> EDKIMSYNAFFWMWVHDMLIDSIKWRDEHGRCINKDKGKTCIKGCNKKCISFQKWVEQKKTEWGKI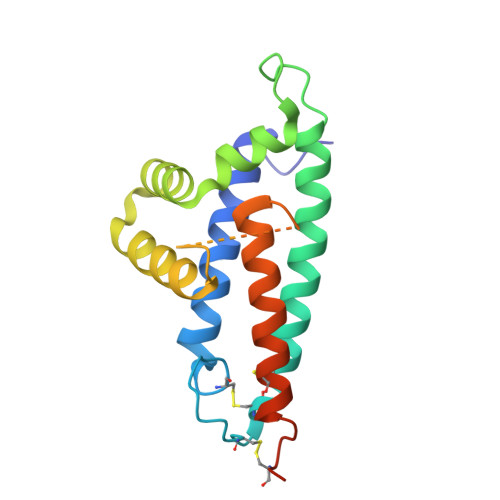KDHFRKQKDIPKDWTHDDFLQTLLMKDLLLEIIQDTYGDANEIKRIEALLEQAGVGGIDFAALAGLYTKGFVAEKDTTIDKLLQHEQKEADKCLKTHTDDTCPPQEDRSVARS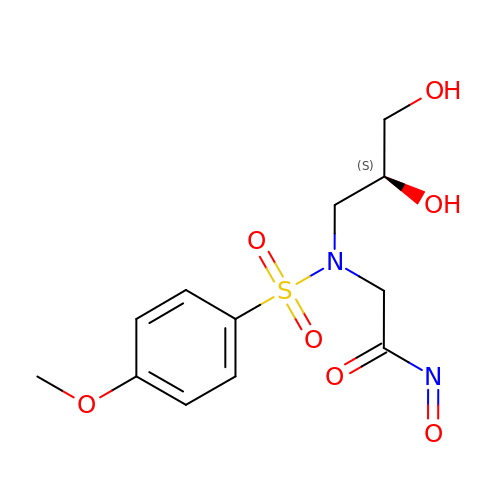2-[[(2S)-2,3-dihydroxypropyl]-(4-methoxyphenyl)sulfonyl-amino]-N-oxo-ethanamide | C12 H16 N2 O7 S | VGUSUBJRLNGCHT-VIFPVBQESA-N The Nedd4 family E3s have nine members in humans (WWP1/2, Nedd4/4 L, Smurf1/2, NEDL1/2, and Itch), which share a common N-terminal domain architecture comprised of a C2 domain and 2–4 WW domains that are responsible for subcellular localization and substrate recognition, respectively. Each HECT-type E3 contains a characteristic HECT domain at its C terminus, which catalyzes the transfer of ubiquitin from E2 to itself and then to the specific substrate. The HECT domain adopts a bilobal structure, in which the E2-binding N-lobe is connected by a flexible hinge loop to the catalytic C-lobe. To prevent excessive ubiquitination of targets and self-destruction by autoubiquitination, HECT-type E3s normally adopt an inactive state characterized by intra- or inter-molecular interaction.

Importantly, key residues involved in the WW2L-HECT interaction (e.g., Met627 in WWP1) are highly conserved in all three proteins. We noticed that Tyr543, the key residue responsible for binding to WW4 in WWP1, is conserved in WWP2 and Itch, which suggests the possibility that the multi-lock autoinhibition mode of WWP1 may be conserved in WWP2 and Itch as well. The GST pull-down experiments further validated this assumption. Although WW2L and LWW34 could interact with HECT, the entire WW region exhibited the strongest binding. In sharp contrast, WW1, WW2, WW34, or L alone could not form a stable complex with HECT. Moreover, when WW in WWP2 robustly interacted with HECT (WT), the Y491AHECT (corresponding to Tyr543 in WWP1) and M575EHECT (corresponding to Met627 in WWP1) mutations, which were predicted to impair packing in WW4-HECT and WW2-HECT, respectively, significantly weakened the interaction between WW and HECT in WWP2, and the Y491A, M575E double mutation completely eliminated the interaction. Accordingly, the W358AWW2 (corresponding to Trp409 in WWP1) and H465AWW4 (corresponding to His517 in WWP1) mutations, which were predicted to impair the packing of WW2-HECT and WW4-HECT, respectively, significantly weakened the interaction between WW and HECT in WWP2, and the W358, H465A double mutation completely disrupted the interaction. Finally, both the Y491A and M575E mutations in WWP2 12L34HECT resulted in elevated ligase activity compared to that of the WT, possibly due to the impaired intramolecular interaction.

> GPGSEFRPLPPGWEKRTDPRGRFYYVDHNTRTTTWQRPTAEYVRNYEQWQSQRNQLQGAMQHFSQRFLYQSSSASTDHDPLGPENLYFQGESGTKQGSPGAYDRSFRWKYHQFRFLCHSNALPSHVKISVSRQTLFEDSFQQIMNMKPYDLRRRLYIIMRGEEGLDYGGIAREWFFLLSHEVLNPMYCLFEYAGKNNYCLQINPASSINPDHLTYFRFIGRFIAMALYHGKFIDTGFTLPFYKRMLNKRPTLKDLESIDPEFYNSIVWIKENNLEECGLELYFIQDMEILGKVTTHELKEGGESIRVTEENKEEYIMLLTDWRFTRGVEEQTKAFLDGFNEVAPLEWLRYFDEKELELMLCGMQEIDMSDWQKSTIYRHYTKNSKQIQWFWQVVKEMDNEKRIRLLQFVTGTCRLPVGGFAELIGSNGPQKFCIDKVGKETWLPRSHTCFNRLDLPPYKSYEQLREKLLYAIEETEGFGQE> ANLKSLPVGDKAPEVVHMVIEVPRGSGNKYEYDPDLGAIKLDRVLPGAQFYPGDYGFIPSTLAEDGDPLDGLVLSTYPLLPGVVVEVRVVGLLLMEDE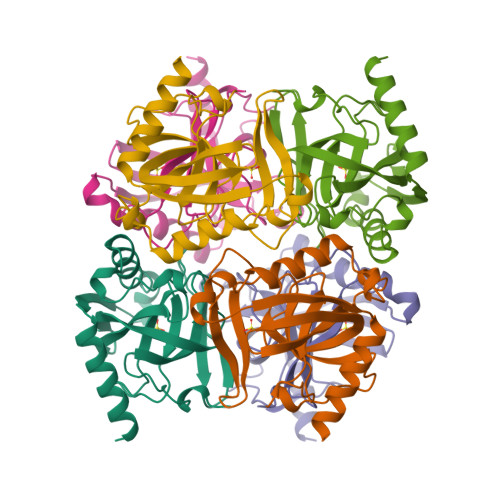KGGDAKVIGVVAEDQRLDHIQDIGDVPEGVKQEIQHFFETYKALEAKKGKWVKVTGWRDRKAALEEVRACIARYKG> ASSVNELENWSKWMQPIPDSIPLARISIPGTADSGTFKLQNPIKQVWGMTQEYDFRYQMDHGARIFDIRGRLTDDNTIVLHHGPLYLYVTLHEFINEAKQFLKDNPSETIIMSLKKEYEDMKGAEDSFSSTFEKKYFVDPIFLKTEGNIKLGDARGKIVLLKRYSGSNEPGGYNNFYWPDNETFTTTVNQNANVTVQDKYKVSYDEKVKSIKDTMDETMNNSEDLNHLYINFTSLSSGGTAWNSPYYYASYINPEIANYIKQKNPARVGWVIQDYINEKWSPLLYQEVI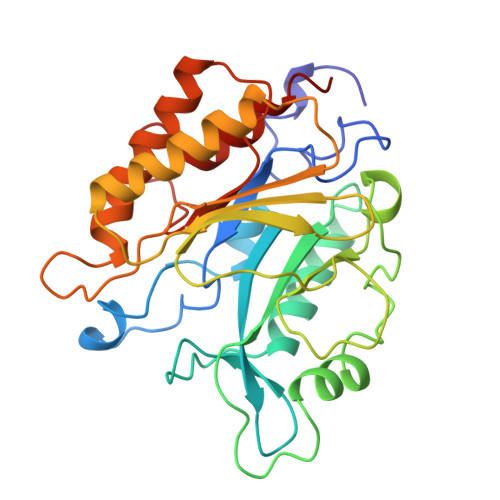RANKSLIKE>MENTENSVDSKSIKNLEPKIIHGSESMDSGISLDNSYKMDYPEMGLCIIINNKNFHKSTGMTSRSGTDVDAANLRETFRNLKYEVRNKNDLTREEIVELMRDVSKEDHSKRSSFVCVLLSHGEEGIIFGTNGPVDLKKIGNFFRGDRCRSLTGKPKLF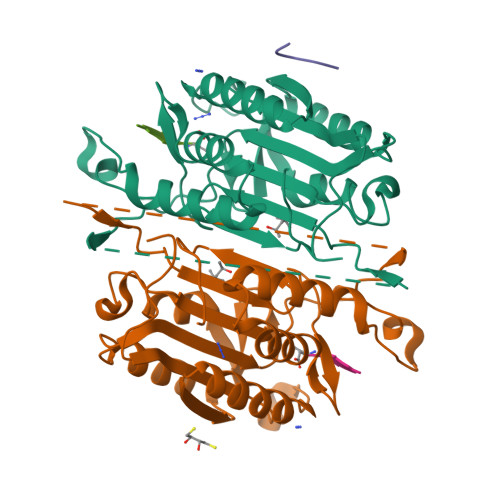IIQACRGTELDCGIETDSGVDDDMACHKIPVEADFLYAYSTAPGYYSWRNSKDGSWFIQSLCAMLKQYADKLEFMHILTRVNRKVATEFESFSFDATFHAKKQIPCIVSMLTKELYFYH[2x];> GVDDD>GMTMPIFNISDDVDLVPAMPAEGRDGGSYRRQIWQDDVENGTIVAVWMAEPGIYNYAGRDLEETFVVVEGEALYSQADADPVKIGPG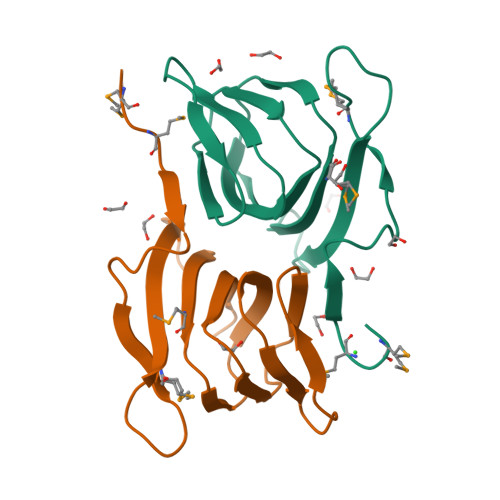SIVSIAKGVPSRLEILSSFRKLATVIPKP[2x]>[2x]GSHMSSLPVPYTLPVSLPVGSCVIITGTPILTFVKDPQLEVNFYTGMDEDSD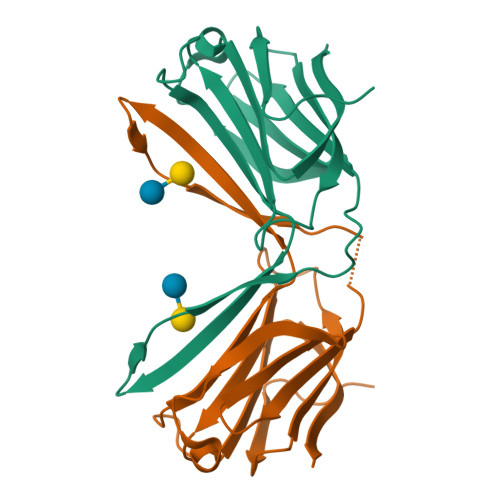IAFQFRLHFGHPAIMNSCVFGIWRYEEKCYYLPFEDGKPFELCIYVRHKEYKVMVNGQRIYNFAHRFPPASVKMLQVFRDISLTRVLISD> NPVENYIDSVLNEVLVVPNIQPSTSVSSHAAPALDAAETGHTSSVQPEDMIETRYVITDQTRDETSIESFLGRSGCIAMIEFNTSSDKTEHDKIGKGFKTWKVSLQEMAQIRRKYELFTYTRFDSEITIVTAAAAQGNDSGHIVLQFMYVPPGAPVPEKRDDYTWQSGTNASVFWQEGQPYPRFTIPFMSIASAYYMFYDGYDGDSAASKYGSVVTNDMGTICVRIVTSNQKHDSNIVCRIYHKAKHIKAWCPRPPRAVAYQHTHSTNYIPSNGEATTQIKTRPD;> SDRLIQITRGDSTITSQDTANAVVAYGVWPSYLTPDDATAIDKPTQPDTSSNRFYTLDSRSWTSASSGWWWKLPDALKNMGIFGENMFYHFLGRSGYTIHVQCNSSKFHQGLLIVAAIPEHQLASATSGNVSVGYNHTHPGEQGREVVPSRTSSDNKRPSDDSWLNFDGTLLGNLPIYPHQYINLRTNNSATLILPYVNAVPMDSMLRHNNWSLVIIPICPLQVQPGGTQSIPITVSISPMFSEFSGPRSKVVF;> SPSAFPYFHPTKEIFIPGQVRNLIEMCQVDTLIPVNNTQENVRSVNMYTVDLRTQVDLAKEVFSIPVDIASQPLATTLIGELASYYTHWTGSLRFSFMFCGSASSTLKLLIAYTPPGVGKPKSRREAMLGTHLVWDVGLQSTASLVVPWVSASHFRFTTPDTYSSAGYITCWYQTNFVVPDSTPDNAKMVCMVSACKDFCLRLARDTNLHTQEG;> NINYFKDAASSGASRLD

Rhinoviruses (RVs) are the main cause of the common cold. Belonging to the large family Picornaviridae, the typical architecture of RVs comprises a ~ 30 nm diameter capsid enclosing a ss(+) RNA genome of about 7200 bases. The building blocks are four capsid proteins (VPs) present as 60 copies each and arranged on a pseudo T = 3 lattice. After the first 3Dstructures of RV-B146 as well as of the closely related poliovirus type 17 had been solved, high-resolution X-ray and cryo-electron microscopy (cryo-EM) structures of numerous RV types and of closely related members of the Enterovirus genus became available and have been used for the design of capsid-binding compounds. These drug candidates attach inside a hydrophobic pocket mainly contributed by amino acid residues of VP1 and displace a natural pocket factor—in most cases a myristate—stabilizing the viral shell against structural changes required for release of the viral RNA genome into the host cell’s cytosol for infection.

Following up on these results we determined the cryo-EM structure of the same RV-A89 in plain buffer lacking OBR-5-340 and DMSO and found that the hydrophobic pocket was filled with myristate. Using the remaining 80% of the particles we solved the structure of the native RV-A89 to a near atomic resolution of 1.76 Å, locally ranging between 1.55 Å and 1.85 Å. Thorough analysis of the hydrophobic pocket revealed an isolated density with elongated shape, which cannot be assigned to a protein chain; it is at the assumed position of a myristate and has its typical shape. Although the full density of the fatty acid appears better visible in a low pass filtered (2.5 Å) map, the density is sharp enough to determine the correct position and orientation of the molecule. The fact that the myristate could not be clearly seen at higher resolution suggests either partial occupancy across the icosahedral virion (i.e. less than the 60 positions would be occupied) and/or loose binding to the hydrophobic pocket. The latter would explain why DMSO readily elutes myristate from its binding site, or why antiviral drug candidates can easily displace the myristate for many rhinovirus types and antivirals. To understand the implication of the missing myristate on the viral conformation, we analyzed the differences of the two atomic models, derived from cryo-EM maps reconstructed from data acquired in the presence or absence of DMSO. However, focused r.m.s.d. analysis of residues forming the hydrophobic pocket revealed a significant conformational change of a five amino acid stretch at the end of the G-H loop corresponding to VP1 residues 218–223 with local average r.m.s.d.Ø of 3.692 Å.We analysed a multidomain xylanase (Xyl) from the hindgut metagenome of the snouted harvester termite Trinervitermes trinervoides that releases xylobiose and xylotriose from beech and birch xylan and wheat arabinoxylan. The four domains of Xyl include an N-terminal GH11 xylanase domain, two family 36-like carbohydrate-binding domains CBM36-1 and 2, and a C-terminal CE4 esterase domain. Instead, individual domains and domain combinations were investigated structurally and for possible interdomain interactions. Xyl exemplifies a “beads-on-a-string” protein where the individual domains are “beads” each connected by a linker (string), with each domain retaining its individual function- making the synthesis of novel super enzymes for rapid and efficient degradation of bio-waste to biofuels within reach.

Xyl bears two family 36 carbohydrate binding modules (CBM) sharing 84% sequence identity. CD spectroscopy revealed CBM36-1 to be folded at 20°C and to retain its fold up to 80°C. CBM36-2, however, was only partly folded at 20°C and completely unfolded at 30°C. CBM36-1 was crystallised in 0.1 M Hepes pH 7.5 and 25% PEG 3000. CBM36-1 consists of 10 β-strands and a short α-helix between the first two β-strands. Eight β-strands form two 4-stranded, antiparallel β-sheets creating a jellyroll structure. Electron density for two metal ions were identified in CBM36-1 and modelled as Ca2+. Metal ion site 1 or Ca2+-1 is adjacent to the sole α-helix, while Ca2+-2 is in a depression at one end of the jellyroll. Ca2+-1 is coordinated by main chain carbonyl oxygen atoms of Gly286 and Asp376, and the side chains of Gln267, Glu269 and Asp376, whereas Ca2+-2 is coordinated by carbonyl groups of Tyr291 and Trp371, and side chains of Asp367 and Asp 372. The pocket is lined with aromatic residues including Tyr277, Tyr293 and Trp371 for substrate binding. The flexible loop Ala366-Asp367-Asn368-Gly369 also contributes to ligand binding.

> GNETIVQCESMTKGGQYTGNINNPFGGVALYGNNDKVSYTQYFASGTHDFTLRGCSNNDNMARVDLKIGGETKGTFYYGGSSPAEYTIKNVNHGTGNQTIELVVTADNGQWDANIDYLKIGGAGVGGNESSGGNQGGNEGNQGGNAGNEGGNQAGNTGNQGGNEGNAGGQHHHHHH(2P,3P,8S)-2-(5-fluoropyridin-2-yl)-6,6-dimethyl-3-(1H-pyrazolo[3,4-b]pyridin-4-yl)-6,7-dihydro-4H-pyrazolo[5,1-c][1,4]oxazine | C19 H17 F N6 O | 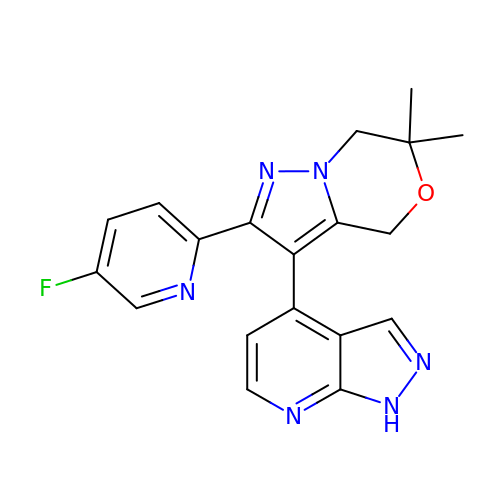WZMIWVZGYMKUDV-UHFFFAOYSA-N CYCLOHEXANE 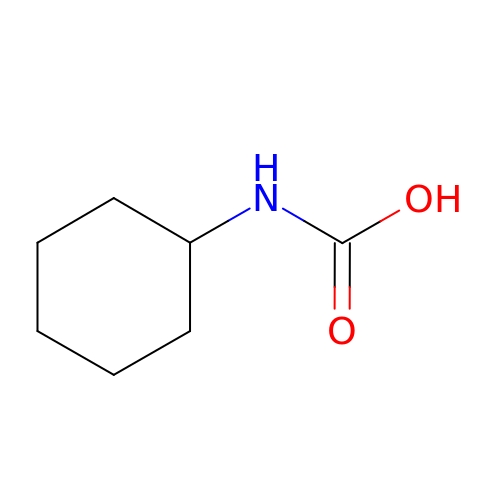AMINOCARBOXYLIC ACID | C7 H13 N O2 | OQQXGCLLMDQESN-UHFFFAOYSA-N An increasing number of surface‐associated proteins identified in Gram‐positive bacteria are characterized by intramolecular cross‐links in structurally conserved thioester, isopeptide, and ester domains (TIE proteins). TEDs are predicted at the distal end of a large number of surface proteins from Gram‐positive bacteria, and the name TIE (thioester, isopeptide, ester) proteins have been introduced for this family. Internal thioester bonds, formed between Cys and Gln side‐chains and first identified in the second thioester domain (TED) of the Streptococcus pyogenes minor pilin Cpa,3 play a negligible role in protein stability, but are suggested to mediate covalent bacterial adhesion. Structures of Bacillus anthracis, vancomycin‐resistant Staphylococcus aureus, and vancomycin‐resistant Enterococcus faecium TEDs show a head domain with Class I topology extended by a β‐sandwich; the latter contributes the thioester bond‐forming Gln via a β‐hairpin insertion into the head domain.

The B. anthracis BaTIE and the 86 kDa E. faecium EfmTIE86 proteins are predicted to comprise a Class II TED as well as three and five CnaB‐type isopeptide domains (IPDs), respectively. EfmTIE86 was identified in genomes of vancomycin‐resistant Enterococcus faecium clinical isolates. SaTIE‐TED (Gln254‐Gly502) and EfmTIE86‐TED (Asp39‐Ala314) were determined by ESI‐MS to be 17 Da lighter than predicted (suggesting the presence of a thioester bond), and readily yielded high‐quality crystals. SaTIE‐TED and EfmTIE86‐TED crystal structures were determined using Se‐SAD phasing and standard refinement procedures. Continuous electron density between Cys and Gln side‐chains either previously shown or predicted to form thioesters (SaTIE‐TED: Cys296 + Gln467,5 EfmTIE86‐TED: Cys88 + Gln292) confirmed the presence of these bonds. Despite pairwise identities of 18–23%, all three Class II TEDs in this study display very similar tertiary structures. With exception of EfmTIE86‐TED Trp146, side‐chains of these residues hydrogen‐bond with the thioester‐forming Cys backbone.

>[4x]GAMGDVTKPTSAKFIETGVKTDGYIRVNMPNHPNEWMISSQFKDSHGNIGYCMDSELPSPTGSGAGSLKYKGAGSDEFYRMFKGGFPSKTAKELGAGNDTEAWYATQLVSWVLAGNFKVSQIVWSHPNHTAAETARVKKAFEKIYDYAKNGKDTPNTEFSITASKTADEGKYHTFTYKTASNKTGNAKLTFTSAKPAGMKIYDADGKEITNNTVKLNSSFTIKVPVTTPSGTLSFKGTANVSTTNPFTFDGRGVYQDAVVMITTSETKDSKSLSAKWTRA[(5R)-5-amino-5-carboxy-7-(4-hydroxypiperidin-1-yl)heptyl](trihydroxy)borate(1-) | C13 H28 B N2 O6 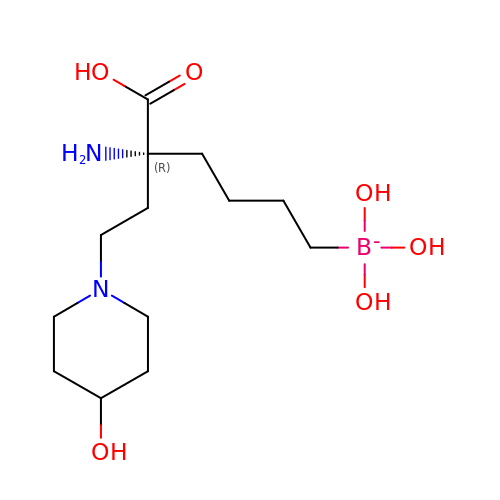| BEHPULZVRPBIEQ-CYBMUJFWSA-N> MATDKEAKDVIDKFIDNVFNFDVLTKERIKEKDEEIKKITTDDMYEKVVYIRPYVGVIQSLNPQHVQYESFSNNGYDIEAELSFRKVSYLVDKGSIPTDSLSTLTVHLVERNQELLIDYFDEIQDVLYGEYMEEEYVFDEDVPLSTILALDLNDNLKSL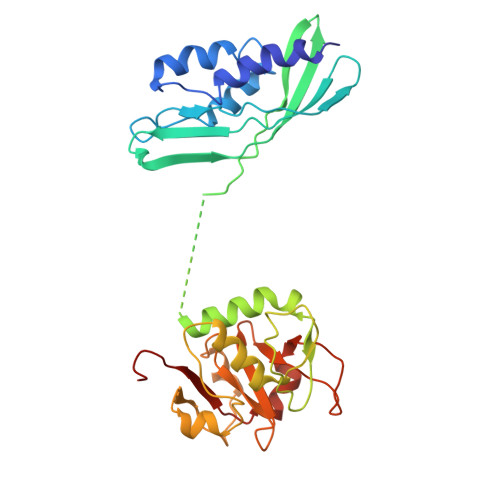SNIKYMFKGAPKENPFGTDKDVYIDTYNLLYWLYLGEDEELAYPMNINYFFTEGRFFTIFGKGHKYKVDVSKFIVGDILFFGRSDTNIGIYVGDGEFISMMGKFPKDETPIGKYKLDDYWNEFNGRVMRFDEEVYI> XS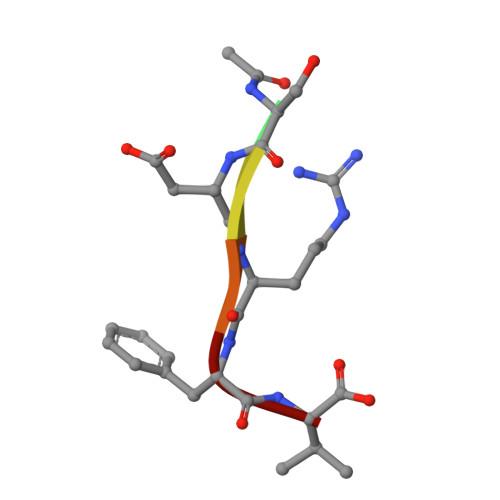DRFV Carbapenemases are enzymes that hydrolyze the carbapenem class of β-lactam antibiotics, rendering the antibiotics in­effective against bacteria that carry carbapenemase genes. With a sequence identity of 91.3% to OXA-48, we expected OXA-436 to have similar characteristics to other OXA-48-like enzymes. The carbapenem-hydrolyzing class D β-lactamase OXA-436 has been characterized as a mesophilic variant of OXA-48, with an observed average thermal stability of 53.8°C and an increased response to changes in temperature when compared with OXA-48.

We solved the crystal structure of OXA-436 to high resolution (1.80 Å) with good overall geometry. Paired refinement, as outlined by Diederichs & Karplus and implemented in the Phenix suite, confirms that the highest resolution shell still contains useful data for refinement with the least-squares target. There are four molecules in the asymmetric unit (chains A–D), and the differences between the chains are localized at surface-exposed polar residues. Chloride ions are observed bridging the dimer interfaces, stabilized by the guanidine group of Arg206 from each chain of the dimers, as has previously been shown for OXA-48, in contrast to the cation-mediated dimerization observed for OXA-10 and OXA-14. In the α3–α4 loop there are two differences: Ala104 in OXA-436 corresponds to Thr104 in OXA-48, and Asp110 in OXA-436 is Asn110 in OXA-48. In the β5–β6 loop, there is only a difference between Val213 in OXA-436 and Thr213 in OXA-48. In OXA-436, a hydrophobic environment with Val213 and Val120 surrounds the R 1 phenyl ring of ampicillin. The ionic interaction of the positively charged R 2 group of imipenem with the side chain of Asp101 in OXA-48 is lost in the modelled complex of imipenem with OXA-436 due to movement of the α3–α4 loop. From the crystal structure of OXA-436 determined to 1.80 Å resolution, we have used molecular dynamics to explore the differences in substrate hydrolysis, with a particular focus on the α3–α4 loop and the β5–β6 loop as tuneable elements for the substrate selectivity of the OXA-48-like group of enzymes.

>[4x]GKEWQENKSWNAHFSEHKTQGVVVLWNENTQQGFTNDLKRANQAFLPASTFKIPNSLIALDLGVVKDEHQVFKWDGQTRDIAAWNRDHDLITAMKYSVVPVYQEFARQIGEARMSKMLHAFDYGNEDISGNLDSFWLDGGIRISATQQIAFLRKLYHNKLHVSERSQRIVKQAMLTEANADYIIRAKTGYSVRIEPKIGWWVGWIELDDNVWFFATNMDMPTAEGLGLRQTITKAVLKQEKIIP>[4x]MASWSHPQFEKGALVPRGSSRFVQDLSKAMSQDGASQFQEVIRQELELSVKKELEKILTTASSHEFEHTKKDLDGFRKLFHRFLQEKGPSVDWGKIQRPPEDSIQPYEKIKARGLPDNISSVLNKLVVVKLNGGLGTSMGCKGPKSLIGVRNENTFLDLTVQQIEHLNKTYNTDVPLV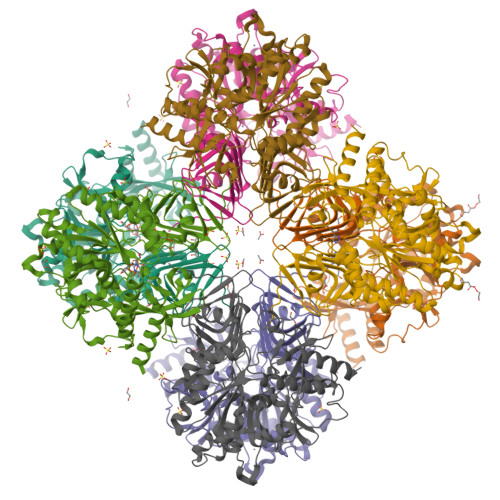LMNSFNTDEDTKKILQKYNHCRVKIYTFNQSRYPRINKESLLPVAKDVSYSGENTEAWYPPGHGDIYASFYNSGLLDTFIGEGKEYIFVSNIDNLGATVDLYILNHLMNPPNGKRCEFVMEVTNKTRADVKGGTLTQYEGKLRLVEIAQVPKAHVDEFKSVSKFKIFNTNNLWISLAAVKRLQEQNAIDMEIIVNAKTLDGGLNVIQLETAVGAAIKSFENSLGINVPRSRFLPVKTTSDLLLVMSNLYSLNAGSLTMSEKREFPTVPLVKLGSSFTKVQDYLRRFESIPDMLELDHLTVSGDVTFGKNVSLKGTVIIIANHGDRIDIPPGAVLENKIVSGNLRILDH>GSMAPLVKNEPQHAKILAIGTANPPNVYHQKDYPDFLFRVTKNEHRTDLREKFDRICEKSRTKKRYLHLTEEMLKANPNIYTYGAPSLDVRQDICNIEVPKLGQEAALKAIKEWGQPISRITHLIFCTASCVDMPGCDFQLIKLLGLDPSVTRTMIYEAGCYAGATVLRMAKDFAENNKGARVLVVCAEITTVFFHGLTDTHLDILVGQALFADGASAVIVGANPEPEIERPLFEIVACRQTILPNSEHGVVVNIREMGFNYYLSGDVPKFVGGNVVDFMTKTFEKVDGKKKDWNSLFFSVHPGGPAIVDQVEEKLGL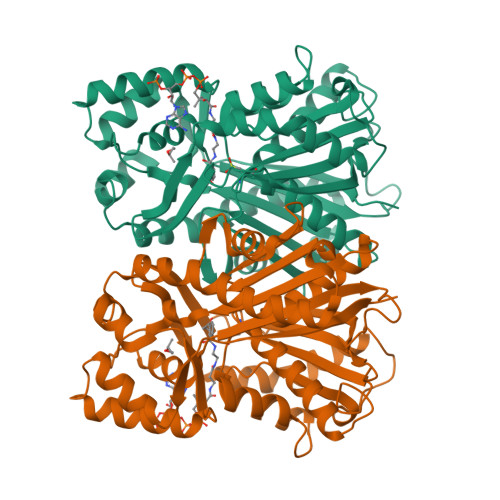KEGKLRATRHVLSEYGNMGAPTVHFILDEMRNKSIEEGKTTTGEGLEWGVVIGIGPGLTVETAVLRSESIRC[2x]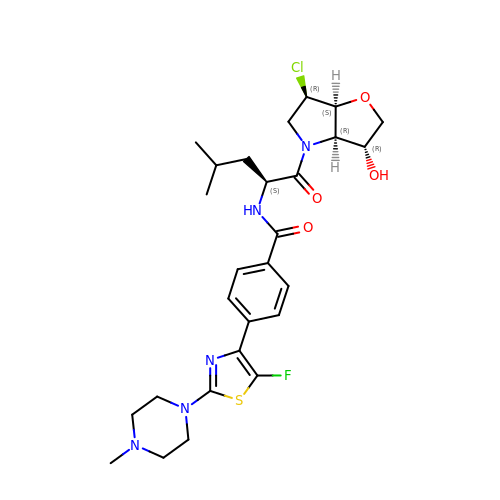~{N}-[(2~{S})-1-[(3~{R},3~{a}~{R},6~{R},6~{a}~{S})-6-chloranyl-3-oxidanyl-2,3,3~{a},5,6,6~{a}-hexahydrofuro[3,2-b]pyrrol-4-yl]-4-methyl-1-oxidanylidene-pentan-2-yl]-4-[5-fluoranyl-2-(4-methylpiperazin-1-yl)-1,3-thiazol-4-yl]benzamide | C27 H35 Cl F N5 O4 S | OXNKTCQYKNTCGL-NBRHSQTJSA-N~{N}-[(3~{S})-2,5-bis(oxidanylidene)pyrrolidin-3-yl]-2,4,6-tris(chloranyl)benzamide | C11 H7 Cl3 N2 O3 | 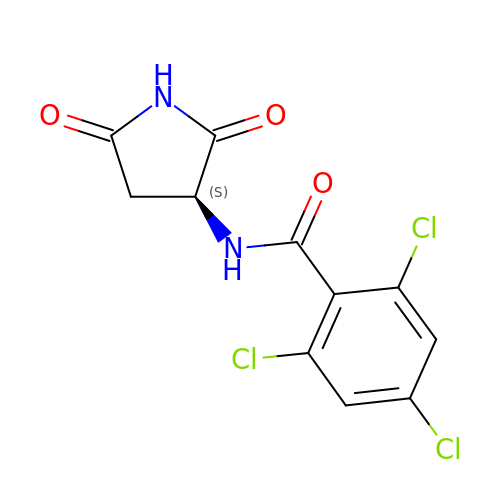LBWIBZYKUVIBKH-ZETCQYMHSA-N>SMGEAICSALPTIPYHKLADLRYLSRGASGTVSSARHADWRVQVAVKHLHIHTPLLDSERKDVLREAEILHKARFSYILPILGICNEPEFLGIVTEYMPNGSLNELLHRKTEYPDVAWPLRFRILHEIALGVNYLHNMTPPLLHHDLKTQNILLDNEFHVKIADFGLSKWRMMSLSQSRSSKSAPEGGTIIYMPPENYEPGQKSRASIK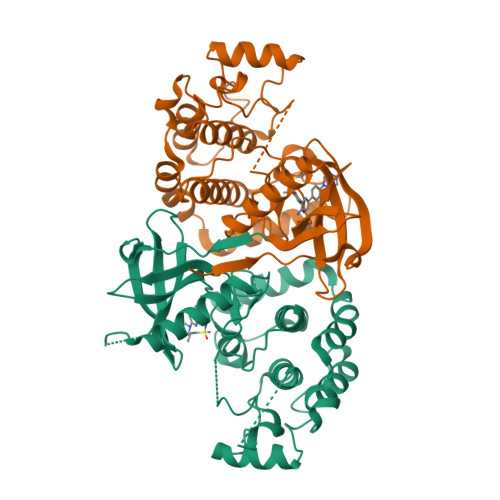HDIYSYAVITWEVLSRKQPFEDVTNPLQIMYSVSQGHRPVINEESLPYDIPHRARMISLIESGWAQNPDERPSFLKCLIELEPVLRTFEEITFLEAVIQLKKTKLQSV[2x]>SSRELIEREASIQAEMRTSMQYVDRTVGKATSIFILDDSKFKGSKQGLTREWSYIGLSADGKKVMNYVWNKQKQDWDVSELGTKSLYNMKLDLEFKTEGAYQDNRLISYNLTGKYPDTNNKLGIDTAISALNTKQVFSKVAKGKKGIAIAYRTDPIQGQMNIAVSFVFDTSGSMDWDLQGRNVKKTGNESRMDILRKKSVIMIKDLAEIGNISVNLVGFSTSAKYIQQNFSNLDNGTNTIIATITKRENLNPDGVTNPGDGLRYGMISLQSQPAQLKYIVLLTDGIPNAYLVDSRALYAGNRVDLSQGAGRVTFNNPIYDLSPTLGYEYSRLGYDLYSRDSITRENSIAYAGEVSKKFGLGIKRVNVIGFSGVNHEIAYGQ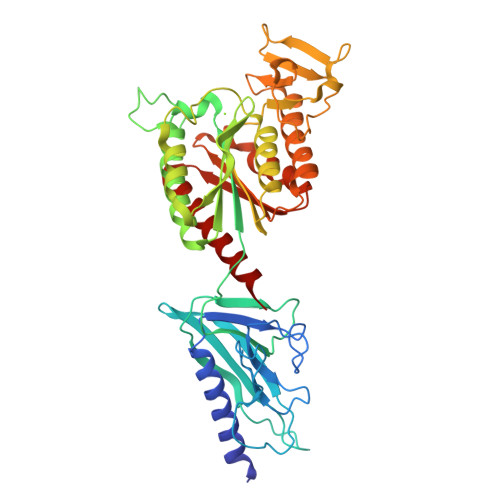SLTDRIGEGGMETKYVSATNEEALQKTFSDIKKQIQQDLWFVSGP[2x]> MNRRVLVTGATGLLGRAVHKEFQQNNWHAVGCGFRRARPKFEQV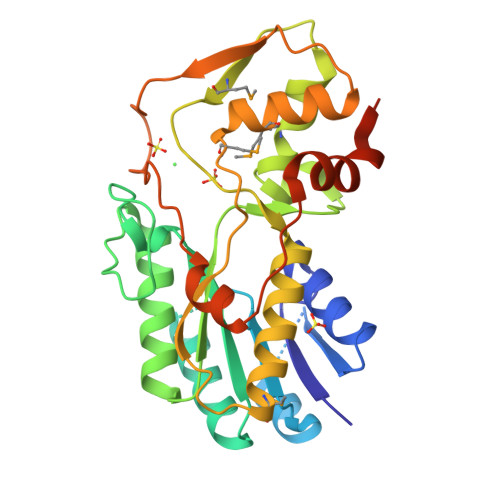NLLDSNAVHHIIHDFQPHVIVHCAAERRPDVVENQPDAASQLNVDASGNLAKEAAAVGAFLIYISSDYVFDGTNPPYREEDIPAPLNLYGKTKLDGEKAVLENNLGAAVLRIPILYGEVEKLEESAVTVMFDKVQFSNKSANMDHWQQRFPTHVKDVATVCRQLAEKRMLDPSIKGTFHWSGNEQMTKYEMACAIADAFNLPSSHLRPITDSPVLGAQRPRNAQLDCSKLETLGIGQRTPFRIGIKESLWPFLIDKRWRQTVFHAENLYFQ> AHHHHHHSSGLEVLFQGPNELNYGQLSISPIFQGGSYQLNNKSIDISSLLLDKLSGESQTVVMKFKADKPNSLQALFGLSNSKAGFKNNYFSIFMRDSGEIGVEIRDAQKGINYLFSRPASLWGKHKGQAVENTLVFVSDSKDKTYTMYVNGIEVFSETVDTFLPISNINGIDKATLGAVNREGKEHYLAKGSIDEISLFNKAISDQEVSTIPLSNPFQLIFQSGDSTQANYFRIPTLYTLSSGRVLSSIDARYGGTHDSKSKINIATSYSDDNGKTWSEPIFAMKFNDYEEQLVYWPRDNKLKNSQISGSASFIDSSIVEDKKSGKTILLADVMPAGIGNNNANKADSGFKEINGHYYLKLKKNGDNDFRYTVRENGVVYNETTNKPTNYTINDKYEVLEGGKSLTVEQYSVDFDS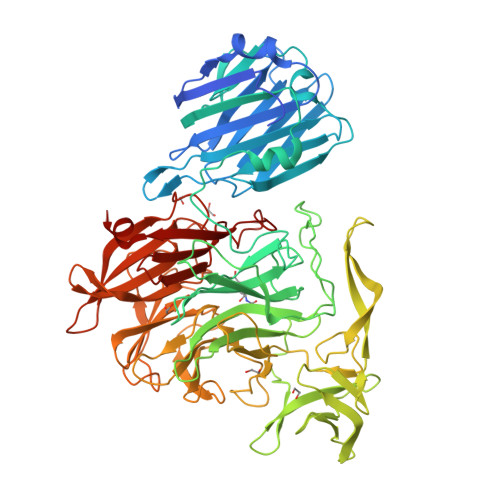GSLRERHNGKQVPMNVFYKDSLFKVTPTNYIAMTTSQNRGESWEQFKLLPPFLGEKHNGTYLCPGQGLALKSSNRLIFATYTSGELTYLISDDSGQTWKKSSASIPFKNATAEAQMVELRDGVIRTFFRTTTGKIAYMTSRDSGETWSKVSYIDGIQQTSYGTQVSAIKYSQLIDGKEAVILSTPNSRSGRKGGQLVVGLVNKEDDSIDWKYHYDIDLPSYGYAYSAITELPNHHIGVLFEKYDSWSRNELHLSNVVQYIDLEINDLTK>[5x]VSPPPPIADEPLTVNTGIYLIECYSLDDKAETFKVNAFLSLSWKDRRLAFDPVRSGVRVKTYEPEAIWIPEIRFVNVENARDADVVDISVSPDGTVQYLERFSARVLSPLDFRRYPFDSQTLHIYLIVRSVDTRNIVLAVDLEKVGKNDDVFLTGWDIESFTAVVKPANFALEDRLESKLDYQLRISRQYFSYIPNIILPMLFILFISWTAFWSTSYEANVTLVVSTLIAHIAFNILVETNLPKTPYMTYTGAIIFMIYLFYFVAVIEVTVQHYLKVESQPARAASITRASRIAFPVVFLLANIILAFLFF

The GLIC is a pentameric 174 kDa (1585 amino acid) membrane protein, characterized by a large extracellular domain that surpasses in size the water channel diameter of most LCPs. The ultra-swollen mesophases were successfully used for the crystallization of a membrane protein, GLIC, with large ECDs otherwise inaccessible to the conventional in meso crystallization method.

GLIC was thus purified in a low-salt/low-detergent buffer that would not disrupt the swollen mesophase during protein reconstitution. Crystallization trials were then setup using three distinct lipidic systems containing 5, 8 and 10 wt% DSPG, yielding highly swollen Pn3m, Ia3d, and Ia3d/Lɑ phases prior to the addition of the crystallization buffer. Protein crystal growth was then consistently observed in all the tested systems and confirmed by means of cross-polarized microscopy, UV microscopy, and single-crystal diffraction, confirming the successful crystallization of GLIC using the in meso approach. Respectively, the crystallization from an initial double-gyroid symmetry (8 and 10 wt% DSPG) yielded crystals after ~7days, whereas crystallization from an initial double-diamond symmetry required slightly longer time (10 days) for crystallization to take place. Single-crystal diffraction experiments from the in meso protein crystals allowed us to resolve the structure of the pentameric membrane protein validating the use of the swollen cubic phases for membrane protein crystallization, thus opening previously unexplored pathways in protein structural biology. The obtained resolution of 6 Å is modest, but typical for first hits of membrane protein crystallization trials. More importantly, in-depth structural analysis revealed that the in meso grown GLIC crystals crystallized in a completely different and unreported space group for this protein, exhibiting a tighter packing arrangement, with less solvent content (56.3% solvent content) compared to loose crystals grown via vapor diffusion techniques (typically 76.7% solvent content). Moreover, the structure obtained from in meso grown crystals shows the GLIC molecules to be in a closed state (see Structure solution and refinement in the Methods section and Supplementary Figure 3), in spite of the presence of H3O+ions at the crystallization pH of 4, which normally stabilize the open state of the channel, as found in the vast majority of reported GLIC structures. The crystals were found to be organized in a different space group compared to crystals of the same protein grown by vapor diffusion, with the noteworthy additional features of tighter packing of the protein and the stabilization of its closed state as opposed to the more conventional open state found in loose crystals obtained by vapor diffusion.> SIPWNLERITPP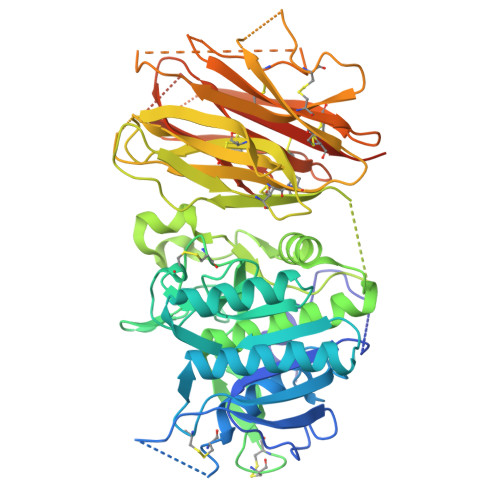RYRADEYQPPDGGSLVEVYLLDTSIQSDHREIEGRVMVTDFENVPEEDGTRFHRQASKCDSHGTHLAGVVSGRDAGVAKGASMRSLRVLNCQGKGTVSGTLIGLEFIRKSQLVQPVGPLVVLLPLAGGYSRVLNAACQRLARAGVVLVTAAGNFRDDACLYSPASAPEVITVGATNAQDQPVTLGTLGTNFGRCVDLFAPGEDIIGASSDCSTCFVSQSGTSQAAAHVAGIAAMMLSAEPELTLAELRQRLIHFSAKDVINEAWFPEDQRVLTPNLVAALPPSTHGAGWQLFCRTVWSAHSGPTRMATAIARCAPDEELLSCSSFSRSGKRRGERMEAQGGKLVCRAHNAFGGEGVYAIARCCLLPQANCSVHTAPPAEASMGTRVHCHQQGHVLTGCSSHWEVEDLGTHKPPVLRPRGQPNQCVGHREASIHASCCHAPGLECKVKEHGIPAPQEQVTVACEEGWTLTGCSALPGTSHVLGAYAVDNTCVVRSRDVSTTGSTSEEAVTAVAICCRSRHLAQASQELQHHHHHH Found in all kingdoms of life, DEAD-box helicase (DDX) is the largest family of RNA helicases that regulate RNA biogenesis by unwinding short RNA duplexes. Like all DDXs, DDX3X contains a helicase core composed of two RecA-like domains (D1D2), harboring 12 highly conserved sequence motifs. The D1D2 core of DDX3X is flanked by N- or C-terminal tails, which are largely unstructured but contain motifs responsible for the unique functions of the subfamily. DDX recognizes short double-stranded RNA (dsRNA) to form a DDX:dsRNA complex; ATP binding to the DDX:dsRNA complex unwinds the RNA duplex, resulting in a complex composed of DDX, single-stranded RNA (ssRNA), and ATP (DDX:ssRNA:ATP).

Here, we report the crystal structure of such a D1D2 core in complex with a 23-bp dsRNA at the pre-unwound state. Our structure shows that the assembly is composed of two D1D2 cores and one RNA duplex (D1D2:dsRNA:D1D2). Crystal symmetry is P31 and the asymmetric unit contains two polypeptide chains (amino acid residues 134–580), two RNA strands (nucleotide residues 1–23 and 4–27, respectively), seven chloride ions, and 72 water oxygens. Our structure of the D1D2:dsRNA:D1D2 complex resembles a clamp that cradles the dsRNA in the middle of four RecA-like domains (two D1s and two D2s). We found no base-specific recognition of RNA by the protein, indicating that the D1D2 core recognizes phosphate backbone and 2ʹ-OH groups only. As highlighted in the zoom-in boxes, NTE residue S181 and D1 residues S183, T201 and R202 recognize nucleotides 11 and 12 in the central region of RNA Strand 1 via hydrogen bonds to both 2ʹ-OH and phosphate backbone of each nucleotide, whereas D2 residues K451, T498, G473, and R480 recognize nucleotides 20, 21, and 22 near the 3ʹ end of the same strand (Strand 1) via hydrogen bonds to phosphate backbone only. We show here that all four domains (NTE, D1, D2, and CTE) recognize 2ʹ-OH groups and thereby discriminate against DNA substrates. We also show that MolA mainly interacts with Strand 1 and MolB mainly interacts with Strand 2. A total of 26 hydrogen bonds formed between the two D1D2 cores and dsRNA to stabilize the pre-unwound complex. Our structure shows that two D1D2 cores jointly reach both terminal ends of a 2-turn, A-form dsRNA, explaining why DDXs, which function in a non-progressive manner, rarely unwind RNA duplexes that are longer than two helical turns.

>[2x]DEDDWSKPLPPSERLEQELFSGGNTGINFEKYDDIPVEATGNNCPPHIESFSDVEMGEIIMGNIELTRYTRPTPVQKHAIPIIKEKRDLMACAQTGSGKTAAFLLPILSQIYSDGPGEALRAMKENGRYGRRKQYPISLVLAPTRELAVQIYEEARKFSYRSRVRPCVVYGGADIGQQIRDLERGCHLLVATPGRLVDMMERGKIGLDFCKYLVLDEADRMLDMGFEPQIRRIVEQDTMPPKGVRHTMMFSATFPKEIQMLARDFLDEYIFLAVGRVGSTSENITQKVVWVEESDKRSFLLDLLNATGKDSLTLVFVETKKGADSLEDFLYHEGYACTSIHGDRSQRDREEALHQFRSGKSPILVATAVAARGLDISNVKHVINFDLPSDIEEYVHRIGRTGRVGNLGLATSFFNERNINITKDLLDLLVEAKQEVPSWLENMAYEHHYKGSSRGRSKSSRFSGGFGARDYRQSSG> G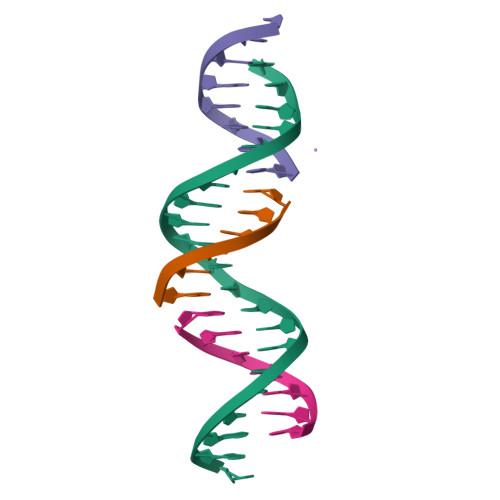AGCAGACCTGACGGCACTCA;> CCGTCA;> TCTGAGTG;> GGTCTGC> ALTCFSEGTKVPAWGCCPASWKSFGSSCYFISSEEKVWSKSEQNCVEMGAHLVVFNTEAEQNFIVQQLNESFSYFLGLSDPQGNNNWQWIDKTPYEKNVRFWHLGEPNHSAEQCASIVFWKPTGWGWNDVICETRRNSICEMNKIYL

The dectin-2 polypeptide contains an extracellular C-terminal C-type carbohydrate-recognition domain (CRD)3 linked to a transmembrane domain and a short N-terminal cytoplasmic domain. Insight into the function of dectin-2 is provided by the demonstration that, although the receptor lacks obvious signaling motifs in the cytoplasmic domain, at the cell surface it is associated with the common Fc receptor γ subunit (FcRγ), which contains an immunotyrosine activation motif that interacts with Syk kinase, initiating signaling that leads to secretion of a range of cytokines. Binding of dectin-2 to a range of pathogens and their surface polysaccharides has been demonstrated. Microbial targets include Candida albicans and other fungi, bacteria such as Klebsiella pneumoniae and Mycobacterium tuberculosis, schistosome egg antigen, as well as dust mites.

The molecular replacement solution revealed that there was one monomer in the asymmetric unit, and difference Fourier maps showed two branches of the Man9GlcNAc2 carbohydrate cross-linking two protein molecules related by a 2-fold symmetry axis. Specifically, the density is strong for seven mannose residues and is fitted well by the Manα1–2Manα1–2Manα1–3(Manα1–2Manα1–3 Manα1–6)Man portion of the oligosaccharide, comprising branches D1 and D2. The carbohydrate was therefore modeled as two symmetry-related molecules each at 50% occupancy. In addition to this set of interactions, which are common to most C-type CRDs that bind mannose and related sugars, C4 and C6 of mannose in the primary binding site make van der Waals contacts with Trp-182. As a result of the orientation being fixed by the interactions with Trp-182 in dectin-2, the mannose residue at the non-reducing terminus occupies a secondary bind site, making hydrogen bonds with Arg-198 as well as contacts with Trp-182 and Val-192. The overall fold of the dectin-2 polypeptide is closely similar to that observed for other C-type CRDs, particularly those from mincle and BDCA-2. Many CRDs, including those in mincle and BDCA-2, bind an auxiliary Ca2+ near the conserved site. However, although several of the amino acid side chains that form ligands for this accessory Ca2+ are present in dectin-2, in the crystals dectin-2 has a Na+ at this site. A more remote Ca2+ is also observed in dectin-2, at a site analogous to a Ca2+ in crystals of mincle and some other C-type CRDs, although no analogous Ca2+ is observed in BDCA-2 crystals.VACV protein N1 is an intracellular virulence factor that is expressed early during infection and modulates innate immunity by at least two strategies: preventing apoptosis and inhibiting NF-κB activation. N1 is a Bcl-2-like protein that contains a surface groove similar to those in cellular anti-apoptotic Bcl-2 proteins that bind the BH3 motif of pro-apoptotic Bcl-2 members. The VACV Bcl-2-like proteins N1, B14 and A52 all form dimers via a common surface comprising alpha helices 1 and 6 (the ‘1–6 face’). Biochemical and structural analysis of these mutants demonstrates that the anti-apoptotic activity of N1 relies on a hydrophobic groove on the surface of the protein and that the anti-NF-κB activity requires an intact dimer interface.

By analogy with VACV proteins A52 and B14, which have the surface groove filled by bulky amino acid residues and do not inhibit apoptosis, we introduced the bulky residue tyrosine at positions R58, Q61 and R71 in an attempt to ‘fill’ the N1 groove and thereby exclude BH3-peptide binding. To determine if the point mutations introduced in N1 generated unanticipated structural changes, R58Y, Q61Y and R71Y N1 were expressed in bacteria, purified to homogeneity and their structures determined at 3.0–3.1 Å resolution. All three mutants crystallized in the same space group as wild-type N1 and the overall structures of all three closely resembled the wild-type protein (0.21–0.39 Å r.m.s. deviation over 108 Cα atoms). For both the R58Y and Q61Y mutants, the tyrosine residue protruded into the groove in a manner likely to reduce BH3 peptide binding. While WT N1 and the groove-filling mutants (R58Y, Q61Y, R71Y) were all dimeric, the I6E mutant was almost exclusively monomeric. Introduction of the groove-filling mutations R58Y and Q61Y abolished the ability of N1 to prevent apoptosis, while mutants R71Y and I6E inhibited STS-induced apoptosis as strongly as WT N1. Investigation of N1 mutant R58Y binding to Bid and Bad was unsuccessful because this mutant bound strongly to all proteins examined, including both pro-apoptotic and anti-apoptotic Bcl-2 proteins and tubulin, for unknown reasons (data not shown). Expression of WT N1 decreased NF-κB activation significantly, as did expression of the groove mutants. However, infection with vN1.R58Y or vN1.R71Y induced lesions that were indistinguishable from vN1.WT. Considering that R58Y N1 was no longer anti-apoptotic and I6E N1 no longer displayed anti-NF-κB activity, our results indicate that suppression of the N1 anti-apoptotic activity does not significantly attenuate VACV virulence whilst suppression of NF-κB activation does.

>[6x]MRTLLIRYILWRNDNDQTYYNDDFKKLMLLDELVDDGDVSTLIKNMRMTLSDGPLLDYLNQPVNNIEDAKRMIAISAKVARDIGERSEIRWEESFTILFRMIETYFDDLMIDLYGEKLEHHHHHH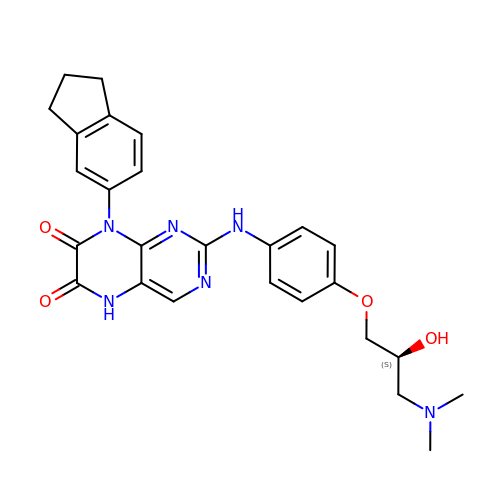8-(2,3-dihydro-1H-inden-5-yl)-2-({4-[(2S)-3-(dimethylamino)-2-hydroxypropoxy]phenyl}amino)-5,8-dihydropteridine-6,7-dione | C26 H28 N6 O4 | FIEBLYFIDPTHGZ-FQEVSTJZSA-N>GSMEKSMSPFVKKHFVLVHTAFHGAWCWYKIVALMRSSGHNVTALDLGASGINPKQALQIPNFSDYLSPLMEFMASLPANEKIILVGHALGGLAISKAMETFPEKISVAVFLSGLMPGPNIDATTVCTKAGSAVLGQLDNCVTYENGPTNPPTTLIAGPKFLATN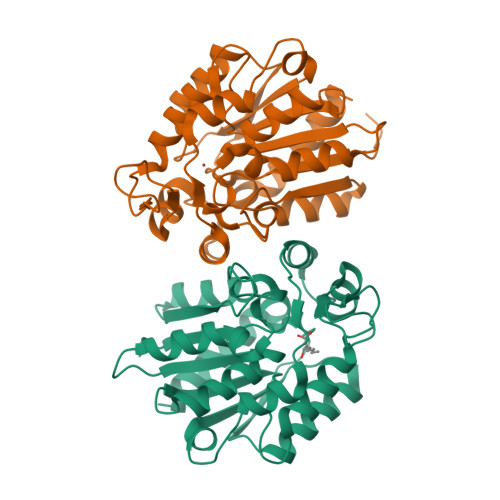VYHLSPIEDLALATALVRPLYLYLAEDISKEVVLSSKRYGSVKRVFIVATENDALKKEFLKLMIEKNPPDEVKEIEGSDHVTMMSKPQQLFTTLLSIANKYK[2x]> GMQLTSENYYSQEANKEYMSVSGYKDFAGTYGKMPCEFYGMEKLNGRWEDEKSTALLVGSYVDSYFEGSLDQFKKDNPEIFTQKGELKANFKQAEEIIARIERDE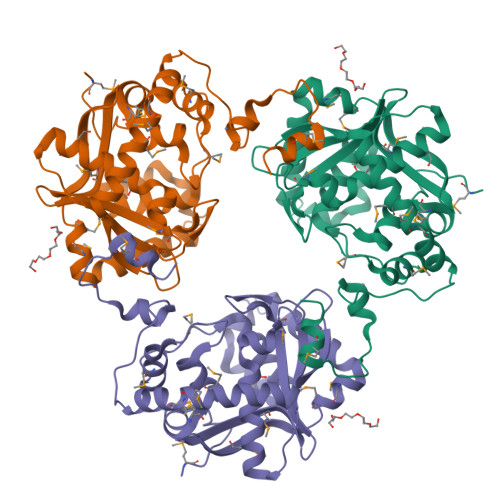YFMKYMSGQKQVIMTGELFGAKWKIKMDSYIPGVAIVDLKVMASITDLKWVKDIGYLDFVRYWGYDIQGAVYQEIVRQNTGEKLPFFIAGATKQTEPDIRIIHVTDNYLQEALHMVEMNMPRILRVKNGEVEPDRCELCDCCRHNRVLKKPISIMDLTAGI>MYFVDRSKIEKTLGFFEHQLALFDSQTDWQSEIGELALQRIGHLLIECILDTGNDMIDGFIMRDPGSYDDIMDILVDEKVVTEKEGDELKK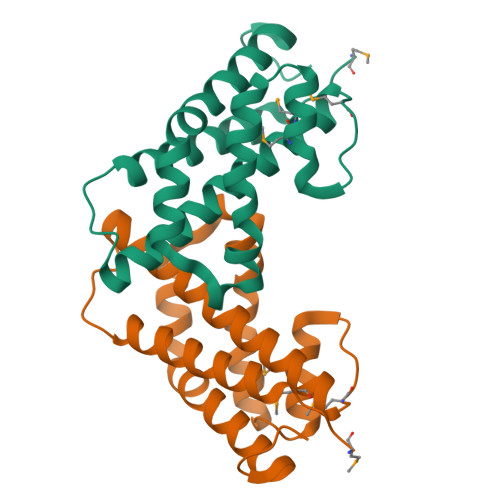LIAYRKTLVQQYLLADSGELYRLIKAHQTALQDFPKRIRSYLETELGPVSAFK[2x]> GMDPNSMSLNDFLSSVLPVSEQFEYLSLQSIPLETHAVVTPNKDDKRVPKS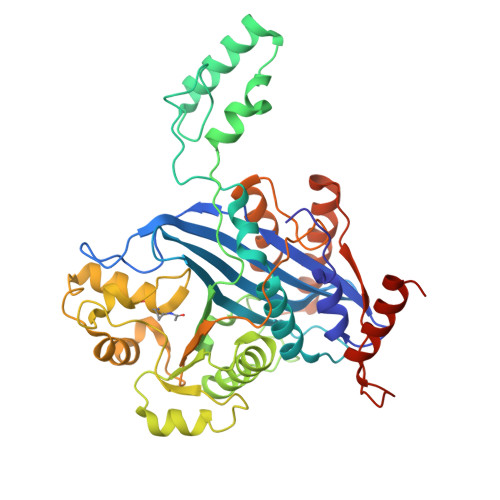TIKTQHFFSLFHQGKVFFSLEVYVYVTLWDEADAERLIFVSKADTNGYCNTRVSVRDITKIILEFILSIDPNYYLQKVKPAIRSYKKISPELISAASTPARTLRILARRLKQSGSTVLKEIESPRFQQDLYLSFTCPREILTKICLFTRPASQYLFPDSSKNSKKHILNGEELMKWWGFILDRLLIECFQNDTQAKLRIPGEDPARVRSYLRGMKYPLWQVGDIFTSKENSLAVYNIPLFPDDPKARFIHQLAEEDRLLKVSLSSFWIELQERQEFKLSVTSSVMGISGYSLATPSLFPSSADVIVPKSRKQFRAIKKYITGEEYDTEEGAIEAFTNIRDFLLLRMATNLQSLTGKREHRERNQPVPASNINTLAITMLKPRKKAKALPKT5-(pyridin-4-yl)-3-[4-(pyrimidin-2-yl)piperazin-1-yl]pyridazine | C17 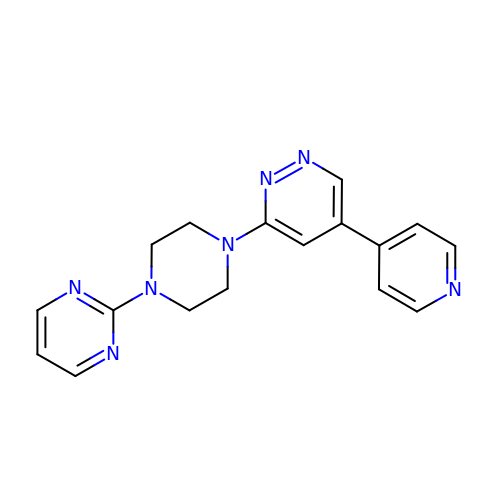H17 N7 | ZCUNPJSEJQKINH-UHFFFAOYSA-N> MGIYRKKDV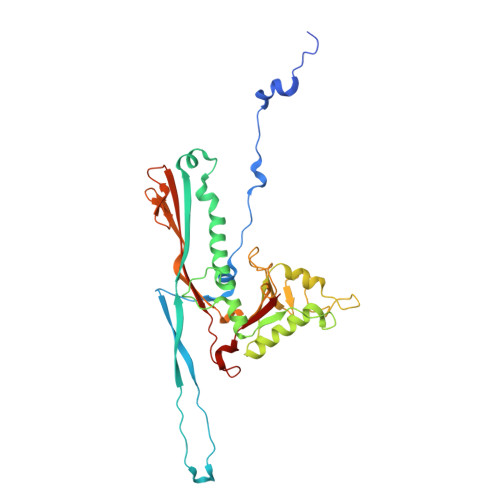IPIPYNNLTSRTDAQALIPEEVSKEMLGKATEQSAVLQQFRRIPVGRNQVRFPVLSALPVAYWVNGDTGLKQTTEINWTNKYLNIEEIATIVPVPDNVLADVDVNVWDEAMPYLIEAFGRTLDSAVVFGTNAPGTFPQAIVPAIAAAGNAVTEGSTAAQGGYLGDLDKAYGKVEEDGFEANGIIAGIGLKGKLRGARDANGQKIDPTRVGADLKSIDGLPVSYPMRGLWPSAGGAGTNVRALVGDWSQFVVGVRQDITLKVLDQAVIQDNTGAIIYNLAQQDMTALRLTFRVGWQVANTLNNDQPTEANRYPAASLIF>[4x]MAIRRPEDFKHYEVQLPDVKIHYVREGAGPTLLLLHGWPGFWWE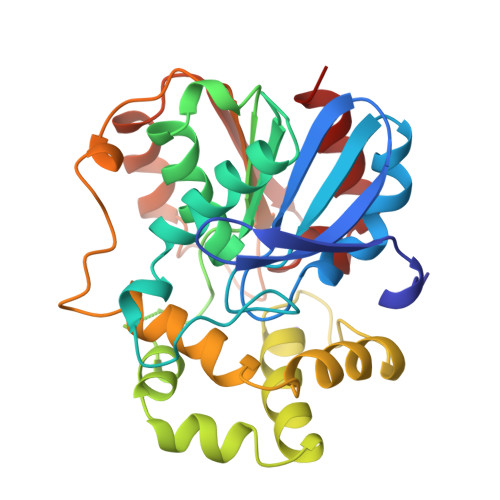WSKVIGPLAEHYDVIVPDLRGFGDSEKPDLNDLSKYSLDKAADDQAALLDALGIEKAYVVGHDFAAIVLHKFIRKYSDRVIKAAIFDPIQPDFGPVYFGLGHVHESWYSQFHQLDMAVEVVGSSREVCKKYFKHFFDHWSYRDELLTEEELEVHVDNCMKPDNIHGGFNYYRANIRPDAALWTDLDHTMSDLPVTMIWGLGDTCVPYAPLIEFVPKYYSNYTMETIEDCGHFLMVEKPEIAIDRIKTAFR>MAKMRISPELKKLIEKYRCVKDTEGMSPAKVYKLVGENENLYLKMTDSRYKGTTYDVEREKDMMLWLEGKLPVPKVLHFERHDGWSNLLMSEADGVLCSEEYEDEQSPEKIIELYAECIRLFHSIDISDCPYTNSLDSRLAELDYLLNNDLADVDCENWEEDTPFKDPRELYDFLKTE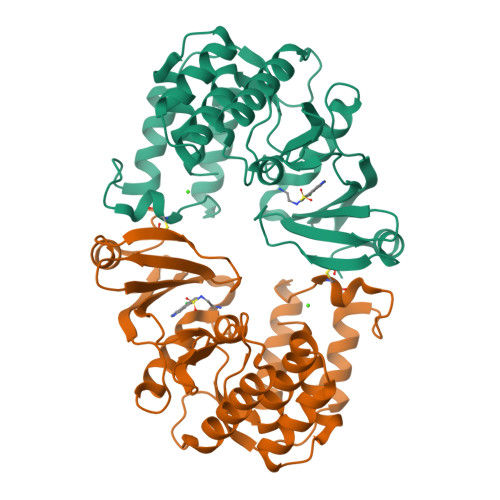KPEEELVFSHGDLGDSNIFVKDGKVSGFIDLGRSGRADKWYDIAFCVRSIREDIGEEQYVELFFDLLGIKPDWEKIKYYILLDELF[2x]>AMGQTVTTPLSLTLGHWKDVERIAHNQSVDVKKRRWVTFCSAEWPTFNVGWPRDGTFNRDLITQVKIKVFSPGPHGHPDQVPYIVTWEALA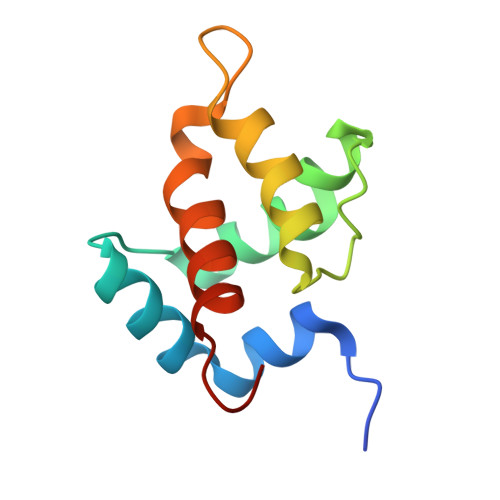FDPPPWVKP[4x]> MRRWHRSLNPALFGERGSGHYFSTTRARLQLQAQDRIICGTHGAGIVAHQTAVNSSDNPMLSSVTTAAPAADLSRTKPHEGTGTSERDPYIRTLHNQRSAAPESSVSQSHTVNAPTVDECEM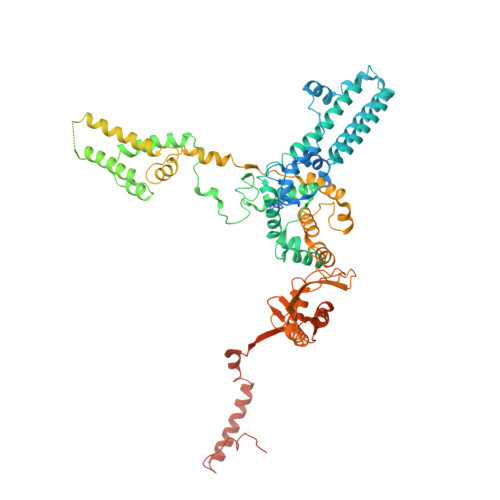LAERWGTMNYWHNDTFPRLVVFLKKLLVPDVSPLSPTAESLLSMFEKVVIPKLTSDEEDRRKLVSLWSETTLQAEAAVTKFLFQRGSFESMLHRIITDALEKMSTLALGGQEGNLALEALKRQTLFKRNDYIQKRLIDVVSNSAYLGYGDSVWQVFFAAVEANEENLLSDRATTDAIRAAWEGVMREDVVRLPDVTGVVALYLTLVCIRESGRLVPEELKELSSGLEDGVRPGVRKLQQYPLIFLHPTVKRRFVVKAVAEILHNSSSNAFSNMLRENGLHDTAREVALCEAMNRNKELAEGDVGDAVGRFVSKGEVKTLLSSLVSGTDAVVRDAVAGIFGIGTTITIDWDAVMQNVDWSNNWQRLATALLSNSAVLSAIVKLVKNAIGAKGMSKHLFTDEYADQLQLILDAREERAASRKQRIENIAQELSSFERVDLSCDLLRKLGVDMTELDTAAAATRNMNVVQRPCIEDGLLSLVLEAVTKRHPNWVKAGVIQTTLKDPFDALRWMMHIFIRLSYVPHAGAATIARLSRRRIGPIGLEPHQFNVPAELGFVEQYDNLQYKRYDWQGWYQRMLDVHNRNVSLRCRICDLQRLDGNGVQFVDMQTERRLRILAQHRVGMGVLKLDADKYEDQADNVTFGTTKLSELLADARKAQLGEEYWPSVELKVRKPSGQSKAHYSLIDNERIEKRSRELYEKYRDAKKRSLFVTPMETWLEVKGMQVRKSVDNADEDGYTLDALQDMMDGDDGDKV Chimeric hybrids derived from the rubredoxins of Pyrococcus furiosus (Pf) and Clostridium pasteurianum (Cp) provide a robust system for the characterization of protein conformational stability and dynamics in a differential mode. A structure design algorithm was applied to the rubredoxins from Pyrococcus furiosus and the mesophilic bacterium Clostridium pasteurianum (Cp) to generate chimeric proteins in which the predicted hybridization interface can preserve each of the interactions in the parental structures. Interchange of the seven nonconserved residues in the metal binding site region between the Cp and Pf A2K rubredoxins yields two complementary hybrid proteins that are accurately represented as a sum of segments from the parental structures. These "cut-and-paste" models match the ultra-high resolution X-ray models to within the structural variability exhibited by the crystallographically nonequivalent molecules in the unit cell.

The coordinates for residues 1–6, 12–38 and 51–54 from Cp rubredoxin were combined with those of residues 7–11 and 39–50 from the Pf protein, to yield the metal binding site-swapped Cp hybrid. The metal binding site-swapped Cp rubredoxin crystallized in a P21 space group with three protein molecules per asymmetric unit, as earlier observed for a V44A variant of Cp rubredoxin. Refinement was extended to higher resolution with inclusion of heavy atom anisotropic temperature factors and all hydrogen atoms, to attain a final R (Rfree) factor of 11.2% (12.5%) for all reflections out to 0.79 Å. The rmsd values for the backbones of the A, B and C monomers with respect to the original search model were only 0.22 Å, 0.24 Å and 0.27 Å, respectively. Molecules A (green) and B (blue) are appreciably more similar to one another than is either of these structures to Molecule C (black). Molecule C diverges most notably from the other three molecules at residues Pro 45, Lys 46 and Ser 47, for which all backbone and sidechain heavy atoms differ by at least 0.5 Å from the superposition with any of the other molecules. Note that the direct interaction between the Lys 46 and Asp 35 sidechains that was predicted in the NMR analysis is indeed observed in the crystal structure. A clear difference between the NMR and X-ray structures occurs at the Glu 50 sidechain, for which the χ1 dihedral angle is 175° in the NMR-derived structure but near +60° in the X-ray structures, despite the fact that the 4.9 Å charge interaction with the Lys 7 sidechain is preserved in both cases. The metal binding site-swapped Cp rubredoxin analysis at 0.79 Å represents the highest resolution Zn2+-form protein structure reported to date. Given the marked similarity in Zn2+ and Fe2+ binding site geometries observed for Cp rubredoxin, the present structure may offer a useful model for the reduced active site as well.

>[3x]MKKYTCKICGYIYNPEDGDPDNGVNPGTDFKDIPDDWVCPICGAPKSEFEEVEE>[4x]MAHHHHHHMKRVGLIGWRGMVGSVLMQRMLEERDFDLIEPVFFTTSNVGGQGPEVGKDIAPLKDAYSIDEL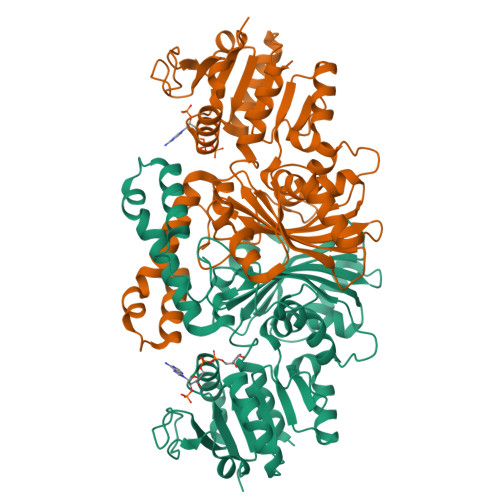KTLDVILTCQGGDYTSEVFPKLREAGWQGYWIDAASSLRMEDDAVIVLDPVNRKVIDQALDAGTRNYIGGNCTVSLMLMALGGLFDAGLVEWMSAMTYQAASGAGAQNMRELLKQMGAAHASVADDLANPASAILDIDRKVAETLRSEAFPTEHFGAPLGGSLIPWIDKELPNGQSREEWKAQAETNKILARFKNPIPVDGICVRVGAMRCHSQALTIKLNKDVPLTDIEGLISQHNPWVKLVPNHREVSVRELTPAAVTGTLSVPVGRLRKLNMGSQYLGAFTVGDQLLWGAAEPLRRMLRILLER> ASSFVTISGT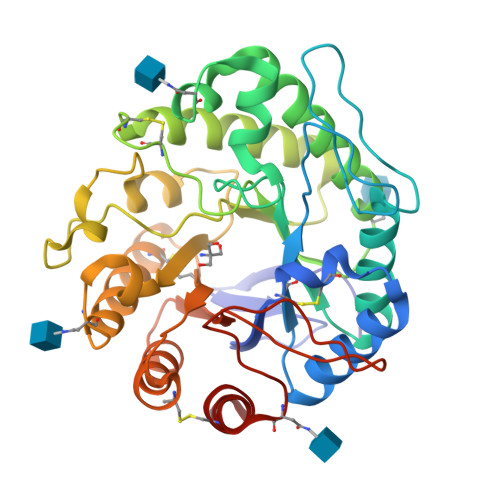QFNIDGKVGYFAGTNCYWCSFLTNHADVDSTFSHISSSGLKVVRVWGFNDVNTQPSPGQIWFQKLSATGSTINTGADGLQTLDYVVQSAEQHNLKLIIPFVNNWSDYGGINAYVNAFGGNATTWYTNTAAQTQYRKYVQAVVSRYANSTAIFAWELGNEPRCNGCSTDVIVQWATSVSQYVKSLDSNHLVTLGDEGLGLSTGDGAYPYTYGEGTDFAKNVQIKSLDFGTFHLYPDSWGTNYTWGNGWIQTHAAACLAAGKPCVFEEYGAQQNPCTNEAPWQTTSLTTRGMGGDMFWQWGDTFANGAQSNSDPYTVWYNSSNWQCLVKNHVDAIN> GPGSMAEEIRTMII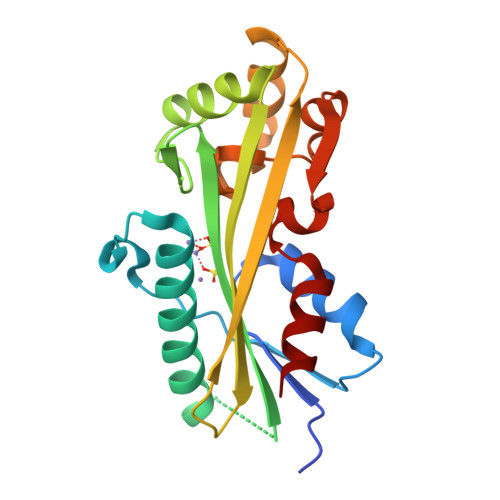GTSSAFRANVLREHFGDRFRNFVLLPPDIDEKAYRAADPFELTESIARAKMKAVLEKARQHSPPISGPAIALTFDQVVVKGDEVREKPLSTEQCRSFIASYSGGGVRTVATYALCVVGTENVLVAHNETETFFSKFGDDIVERTLERGACMNSAGGLVVEDEDMSRHVVRIVGTSYGVRGMEPAVVEKLLSQL> SPNVEACGYSDRVQQITLGNSTITTQEAANAVVCYAEWPEYLPDVDASDVNKTSKPDTSVCRFYTLDSKTWTTGSKGWCWKLPDALKDMGVFGQNMFFHSLGRSGYTVHVQCNATKFHSGCLLVVVIPEHQLASHEGGNVSVKYTFTHPGERGIDLSSANEVGGPVKDVLYNMNGTLLGNLLIFPH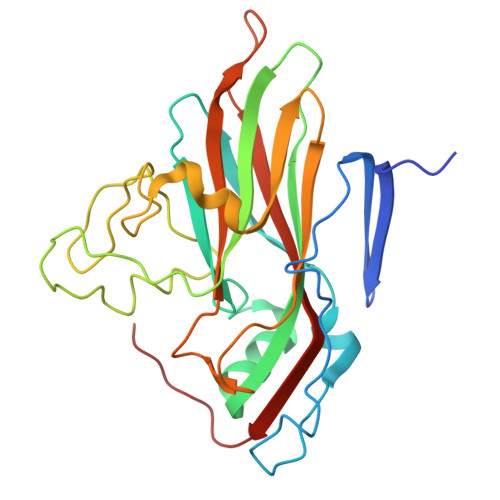QFINLRTNNTATIVIPYINSVPIDSMTRHNNVSLMVIPIAPLTVPTGATPSLPITVTIAPMCTEFSGIRSKSIVPQ> KKRLTESQFQEAIQGLEVGQQTIEIARGVLVDGKPQATFATSLGLTRGAVSQ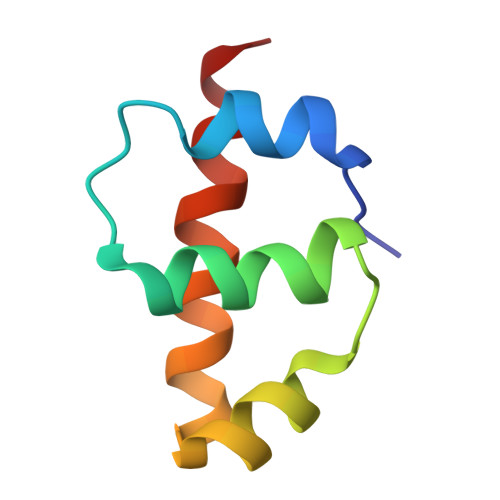AVHRVWAAFEDKN>[2x]MAEQVKPAGVKPKGTVPPPKGNAPAPKANGAPGGASVIKEQDAAKMRRFLFQRTETRSTKWYQIFDTEKLDDEQVVGGHLALLGVLGFIMGIYYISGIQVFPWGAPGFHDNWFYLTIKPRMVSLGIDTYSTKTADLEAAGARLLGWAAFHFLVGSVLIFGGWRHWTHNLTNPFTGRCGNFRDFRFLGKFGDVVFNGTSAKSYKEALGPHAVYMSLLFLGWGIVMWAILGFAPIPDFQTINSETFMSFVFAVIFFALGIYWWNNPPNAAIHLNDDMKAAFSVHLTAIGYINIALGCIAFVAFQQPSFAPYYKELDKLVFYLYGEPFNRVSFNFVEQGGKVISGAKEFADFPAYAILPKSGEAFGMARVVTNLIVFNHIICGVLYVFAGVYHGGQYLLKIQLNGMYNQIKSIWITKGRDQEVQVKILGTVMALCFATMLSVYAVIVWNTICELNIFGTNITMSFYWLKPLPIFQWMFADPSINDWVMAHVITAGSLFSLIALVRIAFFAHTSPLWDDLGLKKNSYSFPCLGPVYGGTCGVSIQDQLWFAMLWGIKGLSAVCWYIDGAWIASMMYGVPAADAKAWDSIAHLHHHYTSGIFYYFWTETVTIFSSSHLSTILMIGHLVWFISFAVWFEDRGSRLEGADIQTRTIRWLGKKFLNRDVNFRFPVLTISDSKLAGTFLYFGGTFMLVFLFLANGFYQTNSPLPPPVSHAAVSGQQMLAQLVDTLMKMIA;> MAEPVENKNQAPAPGAKVPPKGAPAAPKAGAPAAPKGPVAPKAGAPAAKTGASAAKQAGKPRLASLGVTLGRSGVRQESALPYVKPKAVPPPKPAAPAAKGAPAPKGAPAAPAAKAAPGAPVAKAAPKAKKHYFIIENLCVGCGLCLDKCPPKVNAIGYKFYGDVQEGGFRCYIDQAACISCSACFSGDECPSGALIEVLPDGEVLDFSYTPPERLDFDLRFLHRFHREAR;>MDKNSNGKLIALAVGGAVLMGALFFSVSFLTGYIPAPNHSAILTPLRSFMGWFLLIFCASIIIMGLGKMSSAISDKWFLSFPLSIFVIVMVMFLSLRVYWEKGRTTTVDGKYIRTTAELKEFLNKPAATSDVPPAPAGFDFDAAKKLVDVRCNKCHTLDSVADLFRTKYKKTGQVNLIVKRMQGFPGSGISDDDAKTIGIWLHEKF[2x];> MQPQLSRPQTASNQVRKAVSGPWSGNAVHKAEKYFITSAKRDRDGKLQIELVPASGRRKLSPTPEMIRRLIDGEIEIYILTTQPDIAIDMNKEIIDMENRYVIDFDKRGVKWTMREIPVFYHEGKGLCVELHNKIYTLDQFFK;>[3x]MALFGSNDVTTAHSDYEIVLEGGSSSWGKVKARAKVNAPPASPLLPADCDVKLNVKPLDPAKGFVRISAVFESIVDSTKNKLTIEADIANETKERRISVGEGMVSVGDFSHTFSFEGSVVNLFYYRSDAVRRNVPNPIYMQGRQFHDILMKVPLDNNDLIDTWEGTVKAIGSTGAFNDWIRDFWFIGPAFTALNEGGQRISRIEVNGLNTESGPKGPVGVSRWRFSHGGSGMVDSISRWAELFPSDKLNRPAQVEAGFRSDSQGIEVKVDGEFPGVSVDAGGGLRRILNHPLIPLVHHGMVGKFNNFNVDAQLKVVLPKGYKIRYAAPQYRSQNLEEYRWSGGAYARWVEHVCKGGVGQFEILYAQ

Upon illumination, the excitation energy is sequentially transferred from the chlorosome BChls through a monolayered baseplate, Fenna-Matthews-Olson (FMO) complexes, and ultimately to a membrane-embedded RC, where charge separation occurs. Because only one gene encodes two copies of the GsbRC core proteins (PscA subunit), the GsbRC has a homodimeric architecture with a symmetric distribution of pigments, suggesting two identical branches of electron transport chains (ETC) that could be equally utilized. Two membrane-associated PscC subunits (cytochrome cz or cyt c551) contain the cytochrome c domain, which mediates electron transfer from the menaquinol/cytochrome c oxidoreductase to the P84026–29. On the cytoplasmic surface, PscB binds two FeS clusters (FA and FB), serving as terminal electron acceptors.

The two-dimensional (2D) particle images were reconstructed into cryo-EM densities with different assembly states: RC-FMO2 (one RC core with two FMO trimeric complexes), RC-FMO (one RC core with one FMO trimeric complex), and RC alone, which showed the varied stoichiometries possible for the RC and FMO complex. The 3D cryo-EM densities of the RC-FMO2 and RC-FMO1 complexes were reconstructed at 3.08 Å and 3.49 Å resolution, respectively. When our RC-FMO1 structure was superimposed with the previous cryo-EM structure, no significant structural differences could be identified. Note that the FMO1 is the one seen in the RC-FMO1 structure as well as in the previous structure. In both RC-FMO2 and RC-FMO1 density maps, the two PscC subunits bind peripherally on both sides of the PscA dimer symmetrically. The cryo-EM density of the C-terminal heme-binding domain was resolved at a low resolution, and only visible at lower contour levels (1.0σ). These two low-resolution envelopes on the RC periplasmic surface can be identified in both our RC-FMO2 and RC-FMO1 densities. The MGDG lipids can be found in the RC-FMO1 structure, but not the BChl-A816 or PscF. PscF and BChl-A816 were not found in the RC-FMO1 or the previous cryo-EM structure, possibly due to their weak association with the complex. Because the PscE is associated with PscC and FMO2 but was lost in the RC-FMO1 or the previous structure, it likely plays an important role in stabilizing the association of PscC and FMO2. The FeS clusters and P840 dimer that drive the ETC in RC-FMO2 are arranged similarly to the RC-FMO1 and the previously reported structure.> MFKAQATFSRYSAAVSLLLLFSGAAQAAPQSITTLPLQPDGENRWRLPAGEYQGQFTIEQPMQLRCEPGAVIQSQGQGSSLLISAPDVLVEGCTLYEWGSDLTAMDSAVFILPAAERAQISNNRMRGPGFGVFVDGTRDVQVIGNEIDGDAGVRSQDRGNGIHLFAVSGARVLHNHVRNARDGIYIDTSNGNHLEGNVIEDVRYGVHYMFANENSLIDNVTRRTRTGYALMQSRKLTVTGNRSEQDQNYGILMNYITYSTITGNFVSDVQRGDTGGDSMISGGEGKALFIYNSLFNTIENNHFEKSSLGIHLTAGSEDNRISGNAFVGNQQQVKYVASRTQEWSVDGRGNYWSDYLGWDRNNDGLGDIAYEPNDNVDRLLWLYPQVRLLMNSPSIEVLRWVQRAFPVIKSPGVQDSHPLMKLPTEKLLTEKQEPTS;>MNAVEIQGVSQRYGSMTVLHDLNLNLGEGEVLGLFGHNGAGKTTSMKLILGLLSPSEGQVKVLGRAPNDPQVRRQLGYLPENVTFYPQLSGRETLRHFARLKGAALTQVDELLEQVGLAHAADRRVKTYSKGMRQRLGLAQALLGEPRLLLLDEPTVGLDPIATQDLYLLIDRLRQRGTSIILCSHVLPGVEAHINRAAILAKGCLQAVGSLSQLRAEAGLPVRIRASGISERDSWLQRWTDAGHSARGLSESSIEVVAVNGHKLVLLRQLLGEGEPEDIEIHQPSLEDLYRYYMERAGDVRAQEGRL[2x];>[2x]MNQVWNIARKELSDGLRNRWLLAISLLFAVLAVGIAWLGAAASGQLGFTSIPAT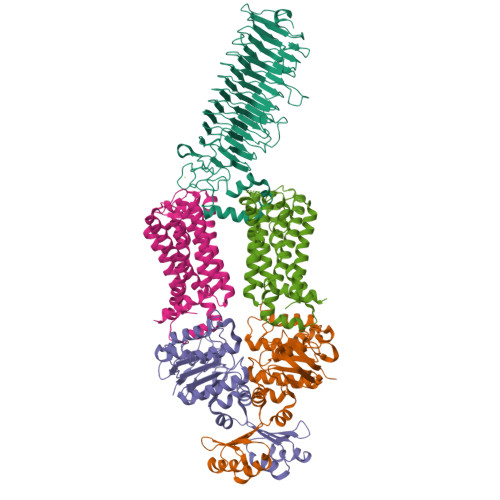IASLASLATFLMPLIALLLAYDAIVGEDEGGTLMLLLTYPLGRGQILLGKFVGHGLILALAVLIGFGCAALAIALLVEGVELGMLFWAFGRFMISSTLLGWVFLAFAYVLSGKVNEKSSAAGLALGVWFLFVLVFDLVLLALLVLSEGKFNPELLPWLLLLNPTDIYRLINLSGFEGSGSAMGVLSLGADLPVPAAVLWLCLLAWIGVSLLLAYAIFRRRLT>MEELREIAERAEADMREISELAEELVEDPVYAVAVRGMALVGAAGVFALGVGGPPEVLEEARRRVEEAAREALRKYEEGADVSELVAELIRETSRQIAEIAEATIKATDDPEVLEEISEFA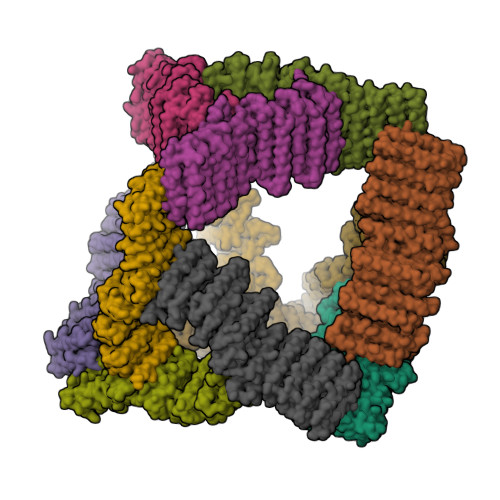EERSRRLSEYAERHVTNPILAATVVALAEVLSAVVRARSYGAPEEVGEKAVKEVREASEEALERYKKGEDVSELVAELIRETSRQIAEIAEATIKATDDPEVLEEISEFAEERSRRLSEYAERHVTNPILAATVVALAEVLSAVVRARSYGAPEEVGEKAVKEVREASEEALERYKEGADESELVAEVMTATAEAVGEIAEATIEATDDPEKRRKIAEFAREKMRRIRELARKLVEDPVLAAAVAARALVLSAAVFAKAYGGPEEYSRLMRRWVEKAAELARRARRLGADESVLVAALMRVAAIAVTAIAMMTVMGVQNAPPEERERILAEATEMIARVLAEATRRVMKRLEDPEAAAELALATIEAITELFVDALEIIRSGEVASRLAKSGIEVIAELAEAAIEHIDDPEQLKKIVKKAAEAIKKIVEELIKKDVEDELLAEVTSEGNRKLSRITSKALTKIKDEKAAAELTIEAIEAITENFLLALERIKDGEVAAKLAEDGLLEIYRLAVSGIEHIDNPEELEKIVKKTEEAVERIVEALEKKDVEPELKEEVEELGKKLVEIVRKLAERKGGSGGSWGHHHHHHG[12x]N-(2-amino-1H-benzimidazol-5-yl)-1-[3-[[(3,5-dimethyl-1,2-oxazol-4-yl)carbamoylamino]methyl]phenyl]-5-hydroxypyrazole-4-carboxamide 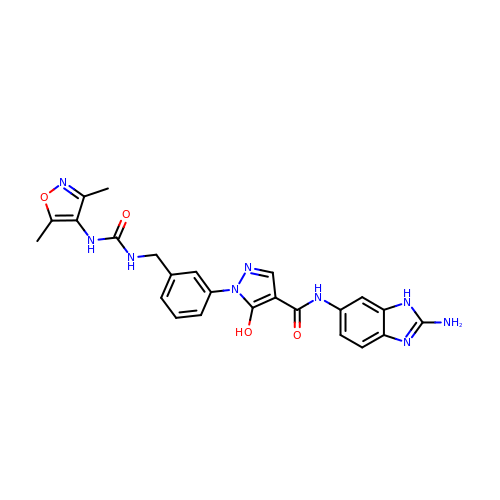| C24 H23 N9 O4 | XUIGQXOFQZKKAN-UHFFFAOYSA-N ethyl (2Z,4S)-4-{[N-(3-methylbutanoyl)-L-phenylalanyl]amino}-5-[(3S)-2-oxopyrrolidin-3-yl]pent-2-enoate 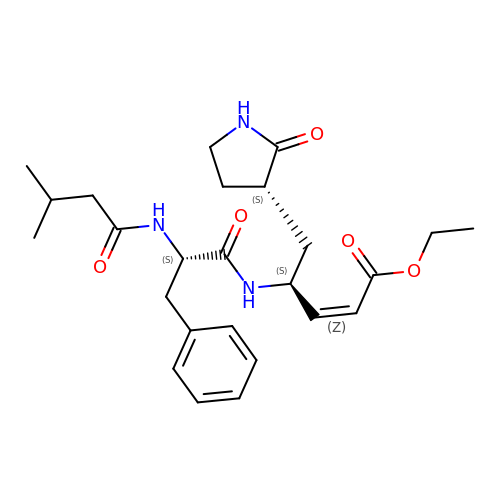| C25 H35 N3 O5 | GTLUNMWXGUIRTC-HBMCJLEFSA-N> QTSVSPSKVILPRGGSVLVTCSTSCDQPKLLGIETPLPKKELLLPGNNRKVYELSNVQEDSQPMCYSNCPDGQSTAKTFLTVYWTPERVELAPLPSWQPVGKNLTLRCQVEGGAPRANLTVVLLRGEKELKREPAVGEPAEVTTTVLVRRDHHGANFSCRTELDLRPQGLELFENTSAPYQLQTFVLPATPPQLVSPRVLEVDTQGTVVCSLDGLFPVSEAQVHLALGDQRLNPTVTYGNDSFSAKASVSVTAEDE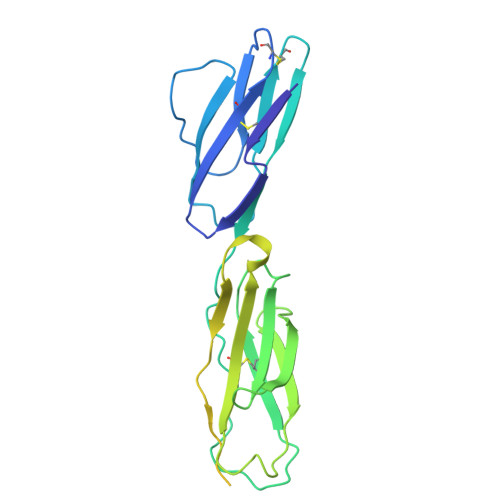GTQRLTCAVILGNQSQETLQTVTIYSFPAPNVILT>ATKEGRVQKYAKERFEALGGLVRKLSYEGRSGAPDLLVILPRGVIWFVEVKKDENTKPDPHQLREHERFRKRGANVFVVGSFKQVDK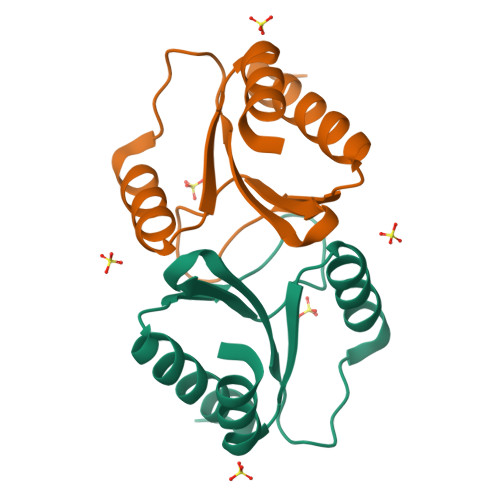LIEHYY[2x]>ADPGTSECSVIGYNAICINRGLHQVPELPAHVNYVDLSLNSIAELNETSFSRLQDLQFLKVEQQTPGLVIRNNTFRGLSSLIILKLDYNQFLQLETGAFNGLANLEVLTLTQCNLDGAVLSGNFFKPLTSLEMLVLRDNNIKKIQPASFFLNMRRFHVLDLTFNKVKSICEEDLLNFQGKHFTLLRLSSITLQDMNEYWLGWEKCGNPFKNTSITTLDLSGNGFKESMAKRFFDAIAGTKIQSLILSNSYNMGSSFGHTNFKDPDNFTFKGLEASGVKTCDLSKSKIFALLKSVFSHFTDLEQLTLAQNEINKIDDNAFWGLTHLLKLNLSQNFLGSIDSRMFENLDKLEVLDLSYNHIRALGDQSFLGLPNLKELALDTNQLKSVPDGIFDRLTSLQKIWLHTNPWDCSCPRIDYLSRWLNKNSQKEQGSAKCSGSGKPVRSIICPTSASLVPR[2x];>[2x]GSAKDPQAIANRFTSNIKGLTQASRNANDGISIAQTTEGALNEINNNLQRVRELSVQATNGTNSDSDLKSIQDEIQQRLEEIDRVSNQTQFNGVKVLSQDNQMKIQVGANDGETITIDLQKIDVKSLGLDGFNVNGPKEATVGDLKSSFKNVTGYDTYAAGADKYRVDINSGAVVTDAVAPDKVYVNAANGQLTTDDAENNTAVDLFKTTKSTAGTAEAKAIAGAIKGGKEGDTFDYKGVTFTIDTKTGDDGNGKVSTTINGEKVTLTVADIAIGAADVNAATLQSSKNVYTSVVNGQFTFDDKTKNESAKLSDLEANNAVKGESKITVNGAEYTANATGDKITLAGKTMFIDKTASGVST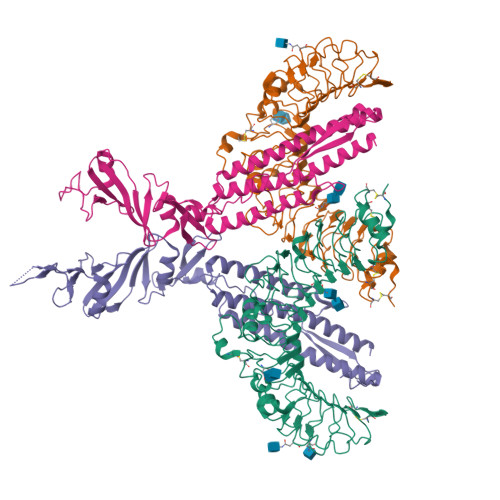LINEDAAAAKKSTANPLASIDSALSKVDAVRSSLGAIQNRFDSAITNLGNTVTNLNSARSRIED>[2x]MGSSHHHHHHSQDPMTVTANQVLRPRGPQIERLTDNRAKVVIEPLERGYGHTLGNALRRVLLSSIPGFAITEVEIDGVLHEYTTVEGLQEDVLDVLLNLKDVAIRMHSGDSATLSLSKQGPGTVTAADIRTDHNVEIINGDHVICHLTKDTALNMRLKIERGFGYQPAAARRRPDEETRTIGRLMLDASFSPVRRVAYAVEAARVEQRTDLDKLVIDIETNGTIDAEEAVRTAADILSDQLSVFGDFTHRDRGAAKPAASGVDPVLLRPIDDLELTVRSANCLKAESIYYIGDLIQKTEVELLKTPNLGKKSLTEIKEVLAQRGLALGMKLENWPPAGVAQHGMLG;> MTSYSFTEKKRIRKDFGKQRSILEVPFLLAIQVDSYREFLQEDVESTKRKDLGLHAALKSVFPISSYSGNAALEYVGYKLGQPVFDERECRQRGMSYGAPLRVTVRLVIYDRESSTKAIKYVKEQEVYLGEIPLMTGNGTFIVNGTERVIVSQLHRSPGVFFDHDRGKTHSSGKLLYSARIIPYRGSWLDFEFDPKDALFTRIDRRRKLPVSILLRALGYNNEEMLAEFFEINTFHINPDEGVQLELVPERLRGETLNFDLADGDKVIVEAGKRITARHVKQLEAAGVAALAVPDDYLVGRILSHDVVDGSTGELLANANDEISEDQLTAFRKAGVDAVGTLWVNDLDRGPYLSNTLRIDPTKTQLEALVEIYRMMRPGEPPTKEAAQNLFHNLFFTFERYDLSTVGRMKFNRRVGRKDVLGESVLYDKKYFAERNDEESKRLVAEHTDTSDILEVIKVLTEIRNGRGVVDDIDHLGNRRVRSVGEMAENVFRVGLVRVERAVKERLSMAESEGLTPQELINAKPVAAAIKEFFGSSQLSQFMDQNNPLSEVTHKRRVSALGPGGLTRERAGFEVRDVHPTHYGRVCTIETPEGPNIGLINSLAVFARTNQYGFLETPYRKVLDGKVSDDVEYLSAIEENEYVIAQANALTDAKNMLTEQFVPCRFQGESLLKPPSEVHFMDVSPMQTVSVAAALVPFLEHDDANRALMGANMQRQAVPTLRSQKPLVGTGIERAVARDSGVTVNALRGGVIEQIDAARIVVKVNEAEIGGGTDAGVDIYNLIKYTRSNQNTCINQRPLVNVGDVIARGDVLADGPSTDIGELALGQNMLIAFMPWNGYNFEDSILLSERVVEEDRYTTIHIEELTCVARDTKLGPEEISADIPNVSEQALNRLDESGVVYIGAEVRAGDIMVGKVTPKGESQLTPEEKLLRAIFGEKASDVKDSSLRVPPGMDGTVIDVQVFTRDGIEKDKRARQIEENEIKRVKKDFDDQFRILEAAIYARLRSQIVGKVANGGANLKKGDSVTDAYLDGLKKSDWFQLRMKDEDAADAIERAQKQIQAHEKEFEARFADKRGKITQGDDLAPGVLKMVKVFLAVKRRIQPGDKMAGRHGNKGVVSNVVPVEDMPYMATGESVDIVLNPLGVPSRMNIGQILEVHLGWAAKGLGRKIQRMLEAQAAVSELRKFLDDIYNHDNAINAQRVDLSQFSDEELLNLGKNLIDGVPMATPVFDGASEAEIKRMLELADLPQSGQTQLYDGRTGEAFDRKTTVGYMHYLKLNHLVDDKMHARSTGPYSLVTQQPLGGKAQFGGQRFGEMEVWALEAYGAAYTLQEMLTVKSDDVQGRNQMYKNIVDGEHEMVAGMPESFNVLVKEIRSLAIHMELEE;> MKDLLNLFNQQRQTLDFDAIKIALASPDLIRSWSYGEVKKPETINYRTFKPERDGLFCAAIFGPIKDYECLCGKYKRMKHRGVVCEKCGTEVTLAKVRRERMGHIDLASPVAHIWFLKSLPSRIGLMLDMTLRDIERVLYFEAYVVTEPGLTPLERRQLLTEEQYLTARQEYNDDFDAAMGAEAVYELLRTIDLQSEM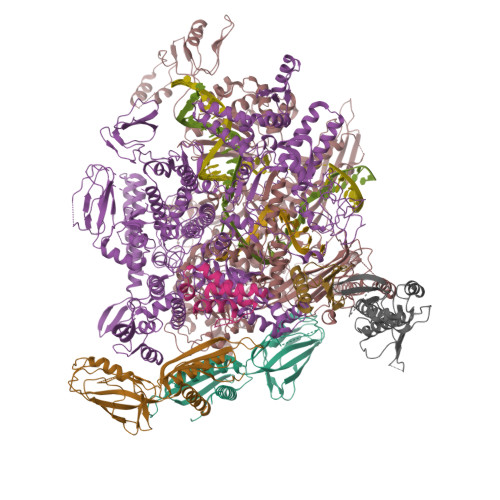TRLREEIASTGSETKLKRLTKRIKLIEAFLESGNRPEWMVMTVLPVLPPDLRPLVPLDGGRFATSDLNDLYRRVINRNNRLRRLLELNAPDIIVRNEKRMLQESVDALLDNGRRGRAITGTNKRPLKSLADMIKGKQGRFRQNLLGKRVDYSGRSVITVGPYLKLHQCGLPKKMALELFKPFVFAKLQRRGLATTIKAAKKLVEREEAEVWDILEEVIREHPVLLNRAPTLHRLGIQAFEPVLIEGKAIQLHPLVCTAFNADFDGDQMAVHVPLSLEAQLEARALMMSTNNILSPANGEPIIVPSQDVVLGLYYMSRALENKKGEGMVFANTSEVKRAYDNRVVELHAKVKVRITQVDVDAVDGKRTSGTSIVDTTVGRALLSEILPEGLPFQLANTEMTKKNISRLINSSYRLLGLKDTVVFADKLMYTGYAYATRAGVSIGIDDMLIPDEKKGILTEAEAEVLEIQEQYQSGLVTAGERYNKVVDIWSRTSERIAKAMMDTIGTEKVENAKGETIDQKSMNSLYIMADSGARGSQAQIRQLAGMRGLMARPDGSIIETPIKANFREGLNVQEYFNSTHGARKGLADTALKTANSGYLTRRLVDVAQDVVITEIDCGTTEGLIMTPIVEGGDVVEPLKERVLGRVVAEDVYLPGNDEEPIVTRNTLLDEAWVAKLEDASVQSVKVRSTISCESSFGVCARCYGRDLARGHQVNIGEAVGVIAAQSIGEPGTQLTMRTFHIGGAASRAAAVDNITVKTTGSVKFNNLKSVAHASGSLVAVSRSGELSVLDGHGRERERYKLPYGATITAKDGDAVKAGQSVANWDPHNHPIVSEVAGFIRFIDFVDGVTVIEKTDELTGLASREITDPKRRGAHAKELRPIVRIVDGKGNDLTIPNTDLPAQYLLPPRSIVNLQDGAAVGVGDVVAKIPQEASKTRDITGGLPRVADLFEARKPKDPAILAERSGIISFGKDTKGKQRLIIKDTDGSEHEELIPKYRQIIVFEGEHVTKGETVVDGEPSPQDILRLLGVEPLAAYLVKEIQDVYRLQGVKINDKHIEVITRQMLRKVEIVDQGNSKFLNGEQVERQRVIEENARLVKRNELPAKYDPVLLGITKASLATESFISAASFQETTRVLTEAAVRGTRDNLRGLKENVIVGRLIPAGTGLAYHAGRRKASGLTDSEMETLSGKPAGAEPVAALADAGADEE;> MARITVEDCLEVVNNRFELVMMASKRARQLANGVQPLIENAAASDKPTVMALREIAARRIDNALIDEVEKAERERAEREALEWAAAEVVADEDMSKNDD;> GAMDMSKELLLVVDAVANEKGVPREVIFDAIEAALASAAKKRYPDQDVLARVTIDHKDGTYETYRRWEVVADDVVMESPDRQVRLMDAIDEADGVDVGDYIEEQIENPDFGRIAAQAAKQVIVQRVREAERQQVVDAWKDRVGELITGVVKRAERGNIFVDLGGNAEAFIPKDKGIPRDVLRPGDRVRGYLAEVRSEPRGPQLFISRAAPEFMIELFKLEVPEVGQGLVEINACARDPGDRAKIAVIAHDARTDPIGACIGMRGSRVQAVSNELNGERVDIVLWNENPANFVINAMAPAEVQSIIVDEDKHSMDLAVAEDRLAQAIGKGGQNVRLASRLTGWQLNVMTADQVAAKSEAEQAAARQLFMDRLEVDEEISAILVSEGFNTVEEIAYVPVGELLAVEGFDEDIVEELRARARDALLNAALAEEEGLEGTQPTEDLLALEGMDEETAVALAEHGVRTSEDLSDLAADEIVDFGIEGLTQERAAALILAARAEEIARLERGE;> GAMAMNEFTQISGYVNAFGSQRGSVLTVKVENDEGWTLVEEDFDRADYGSDPEFVAEVSSYLKRNGGIKDLTKVLTR>ISEFARAQLSEAMTLASGLKTKVSDIFSQDGSCPANTAATAGIEKDTD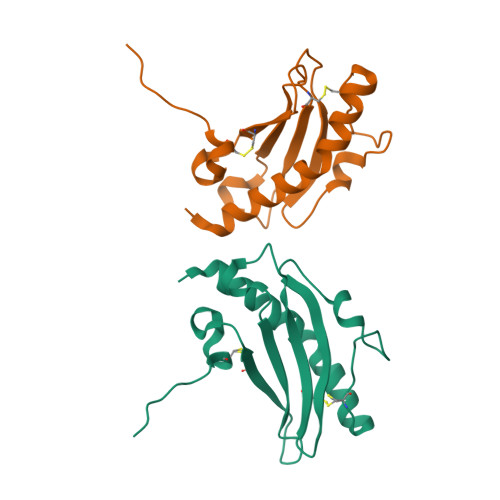INGKYVAKVTTGGTAAASGGCTIVATMKASDVATPLRGKTLTLTLGNADKGSYTWACTSNADNKYLPKTCQTATTTTP[2x]DEPRENYL | C13 H19 N | 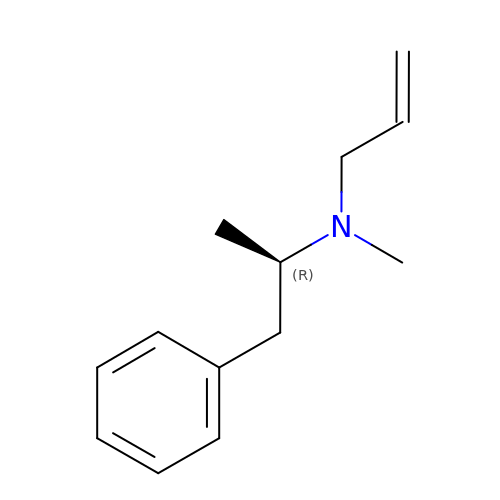BVYBGDRWIWQPOV-GFCCVEGCSA-N>[6x]MISQSRYIRIISGVGAAAPVAGRKLILRVMTTNNVIPPGIVIEFDNANAVLSYFGAQSEEYQRAAAYFKFISKSVNSPSSISFARWVNTAIAPMVVGDNLPKTIADFAGFSAGVLTIMVGAAEQNITAIDTSAA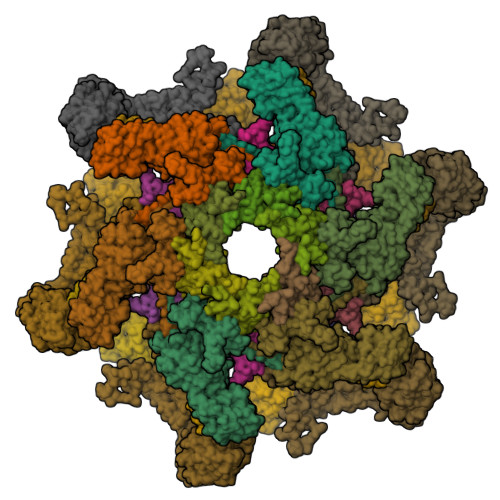TSMDNVASIIQTEIRKNADPQLAQATVTWNQNTNQFTLVGATIGTGVLAVAKSADPQDMSTALGWSTSNVVNVAGQSADLPDAAVAKSTNVSNNFGSFLFAGAPLDNDQIKAVSAWNAAQNNQFIYTVATSLANLGTLFTLVNGNAGTALNVLSATAANDFVEQCPSEILAATNYDEPGASQNYMYYQFPGRNITVSDDTVANTVDKSRGNYIGVTQANGQQLAFYQRGILCGGPTDAVDMNVYANEIWLKSAIAQALLDLFLNVNAVPASSTGEAMTLAVLQPVLDKATANGTFTYGKEISAVQQQYITQVTGDRRAWRQVQTLGYWINITFSSYTNSNTGLTEWKANYTLIYSKGDAIRFVEGSDVMI;>KIPLTAVPNQAISFNAGSSYWKIRLYQNMDMMNADISRDGVIVCHGVRCFGGIPLLQYSHQYRPDYGNFVFDRDADWTLFGDGINLFYLDGAEFAEYQALAT[6x];>[6x]STSTIRTGTNNDILLDDNGNMVILRDVEACAQDVRAAMLMRTGENIFDVNSGVGYFEYIFSPQKSYDDARKSIADAILSSPDVTGIEQLDIDITGEVFGVDAKVITIH;>[6x]MINVSGFGTGIVIVSASSFPMGFSLSKFADDESPISSKELEPFGYEMLYDGGLFAFDKAAPLEVSVSVIAGSEDDINLRILLNSKKGSFRFLPGIIPDMTTLVATLPDGGRTVLSNGTILKGPAIDTIQNTGRRKGNTYTFVFGSYLGAQTA;>MANYNYIVDTGVIVADTADVLSDVEAEFRAALGANINLAASTPQGSLVAAEAIARSSVMRNEARIANTINPNVSFGTFLDAICALMGIERGSDLSTFGYGVQVTGRSQTRISTGSRVQTPAGAIFTVMSDVTIPAGGVATIDIKSQEYGNIPLPVGNLIIIDGTIGWSGAKVIASTRVDPGSRQMSDAELKNARVNRLAIQGRNSTMAIKAYVSAVPNVTSVNVIENNTGAVQVVNGVSFTLPYAVWVCVAGNPDKQAVADALWAAHNGGTPWDYGATNNGVPVDGPNGVPVRDPASGRKYVVKWTTPIMYDGYVNVTVQQGSSSVAPEAIQNAVVNYAQGKVEGEEGLVVGASLSAFEVAGAIAREIPGIYIKLCQVACVAAGSPAPAPGDFTSEYVMSAFGQATISVGNVRVTFV[6x];>LPAYNSDIQQALKWLHNQAPGITGLIQRKAQWYDRFSRQFWANWERDVFHLKTANPFGLMVWCIILGTPSKGFGLYPKNSSWAFGRLRQNFIYSGTQVPPPADASPGGNFYGGGNAEILNLDEIRKVLQLRYVALISNGSIAYINRMLRYIFNDDEPWDEATGLYFYLMDSTGENGPVENLAVYRKDWEGMVLLSSSPRTNHVLTSTPASDADWPGVDPAASGIPVTVETASATAPDGSATVCKLTKPAGSTAYVSAPIDGPLGSGSTVTFSFFAKAGSTRFIAIQSAADFPSRADAVFDLDSGNVISDQMLDSSVVSARMIRLENGWWRCVLTTKTVSSSFRAAYVAPAETNFSWIDSNSSAAIDVLIWGAQIELGDTPTGYLKTTGAPVTITDYVLQNAQTGTVKFTQPLPTGVEAYWTGDWKGGTAAEPARFAVGNGTQDTFTLSDPAYIGLPTSGAFKLEYRVGPALNLSPQLINLMNDRAVGIMPTCAGCDVKVI[6x]Sdk1 and Sdk2 are single-pass transmembrane proteins, with extracellular regions composed of 6 N-terminal immunoglobulin (Ig) domains followed by 13 fibronectin type III (FNIII) domains, and a relatively short intracellular domain terminating in a Postsynaptic density/Discs Large/ZO-1 (PDZ) binding motif. Here, we report the crystal structures of cell-cell adhesive homophilic dimers of mouse Sdk1 and Sdk2, each mediated by the four N-terminal Ig domains. These four domains adopt a horseshoe conformation, like many other IgSF cell-cell recognition proteins, but they interact in a unique back-to-back anti-parallel manner not previously observed. Overall, our data suggest a model in which Sdks form cis dimers on isolated cell surfaces, which dissociate to form trans dimers through the same interface when contact is made to a cell surface expressing the cognate Sdk.

The N-terminal four Ig domains of both Sdk1 and Sdk2, and the chimeric construct, Sdk2Ig1–2/Sdk1Ig3–4, are arranged in highly similar horseshoe structures, with pairwise root mean square deviations over aligned Cα atoms (RMSDs) among all protomers of 2.4 Å or less. Two non-overlapping interfaces hold the horseshoe together: a conserved and relatively rigid Ig1:Ig4 interface and a more flexible and varied Ig2:Ig3 interface. These intramolecular interactions bury extensive combined intramolecular surface areas of 2620 Å2 in Sdk1, 2459 Å2 in Sdk2 and 2567 Å2 in the Sdk2Ig1–2/Sdk1Ig3–4 chimera, implying that the horseshoe should be a stable element in all of these molecules. Remarkably, the Sdk2Ig1–2/Sdk1Ig3–4 chimera structure features the same set of hydrogen bonds and hydrophobic interactions that mediate both Ig1:Ig4 and Ig2:Ig3 interfaces. A Sdk2Ig1–2/Sdk1Ig3–4 chimera was well behaved and formed a strong dimer in solution with comparable affinity to Sdk1Ig1–4 and Sdk2Ig1–4. Interestingly the Sdk2Ig1–2/Sdk1Ig3–4 chimera had a dimerization affinity intermediate to that of Sdk1 and Sdk2, suggesting that the Sdk2 Ig1–2 contributions to dimer affinity may be more than Sdk1 Ig1–2 while the Sdk1 Ig3–4 contributions to dimer affinity may be less than Sdk2 Ig3–4, and could therefore both underlie the lower dimer affinity of Sdk1 relative to Sdk2. The crystal structure of this chimera did not show an interaction between Ig3–4 regions in the dimer, although given the variability observed in the conformations of the dimers in the different Sdk1 and Sdk2 crystal structures, the Ig3–4 regions may interact in solution. Sdk2Ig1–2/Sdk1Ig3–4 behaved more like Sdk2 than Sdk1 in the SPR assay: It bound to the Sdk1Ig1–6 surface similarly to Sdk2Ig1–4, and more tightly to the Sdk2Ig1–6 surface than Sdk1Ig1–4 although not to the same level as Sdk2Ig1–4. These results suggest that the majority of the Sdk1/Sdk2 specificity is localized to Ig1–2, but that Ig3–4 may also contribute to specificity.

>GPAGAQDDVPPYFKTEPVRTQVHLEGNRLVLTCMAEGSWPLEFKWLHNNRELTRFSLEYRYMITSLDRTHAGFYRCIVRNRMGALLQRQTEVQVAYMGSFEEGEKRQSVNHGEAAVIRAPRISSFPRPQVTWFRDGRKIPPSSRIAITLENTLVILSTVAPDAGRYYVQAVNDKNGDNKTSQPITLAVENVGGTHEAMAPIIVVAPGNRSVVAGSSETTLECIANARPVEELSVHWKRNGVRLTSGLHSYGRRLTITNPTSADTGMYVCEATLRGSTFEPARARAFLSIIEPPYFTAEPESRILGEVEETMDIPCRAMGVPLPTLQWYKDAVPLSKLQNPRYKVLPSGGLHIQKLSPEDSGIFQCFASNEGGEVQTHTYLDVTN[2x]>[4x]GINDLDISPIDPQTGGSFDQQGVFVKGYAMLGVTGQKGIDGSPDLDGQDEGESGFYRTTFNCNELPTDECLWAWQKNQDIPQLTSISWSPSSQRTEWVYVRLGYDITQYNFFLDQTEGMTDAETLRQRAEIRFLRALHYWYFLDLFGKAPFKEHFSNDLPVEKKGTELYTYIQNELNEIEADMYEPRQAPFGRADKAANWLLRARLYLNAGVYTGQTDYAKAEEYASKVIGSAYKLCTNYSELFMADNDENENAMQEIILPIRQDGVKTRNYGGSTYLVCGTRVAGMPRMGTTNGWSCIFARAAMVQKFFSNLEDVPMLPADVEIPTKGLDTDEQIDAFDAEHGIRTEDMIKAAGDDRALLYSGVGGGRRKIQTDAISGFTDGLSIVKWQNYRSDGKPVSHATYPDTDIPLFRLAEAYLTRAEAIFRQGG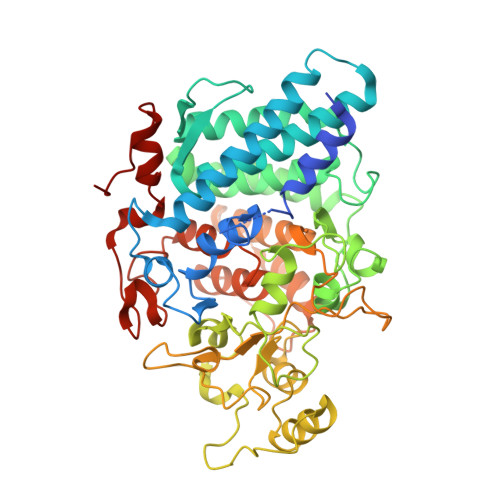DATGDINELRKRANCTRKVQTVTEQELIDEWAREFYLEGRRRSDLVRFGMFTTNKYLWDWKGGAMNGTSVASYYNKYPIPVSDINNNRNMSQNEGYK>MFNSVLDTIGNTPLIRLSKASELTGCDIYGKAEFLNPGQSVKDRAALYIIRDAEKRGLLRPGGVIVEGTAGNTGIGLTMVAKALGYRTAIVIPETASQEKKDALRLLGAELIEVPAAPYRNPNNAVRLSGRLAEQLAKTEPNGAIWANQFDNTVNRQAHIETTAQEIWRDTSDQIDGFVAAVGSGGTLAGTAIGLKERNHNIKIALADPHGAALHAFYTTGELKAEGDSITEGIGQGRITANLEGFTPDFSYQIPDAEALDILFALVEEEGLCLGGSSGI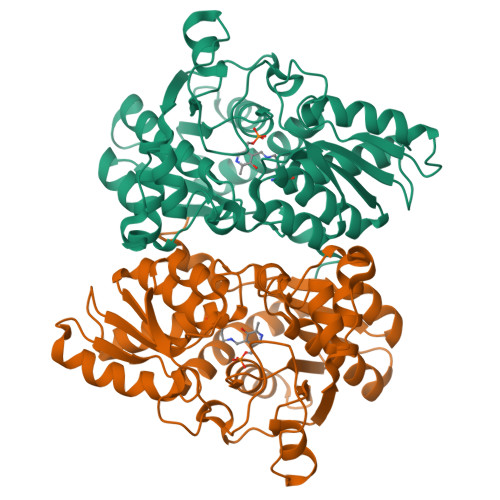NIAGAIRLAKDLGPGHTIVTVLCDYGNRYQSKLFNPAFLRGKSLPVPRWLEKKTEIDIPFEG[4x]> GPLGSSATPREDFRVRCTSKRAVTEMLQLCGRFVQKLGDALPEEIREPALRDAQWT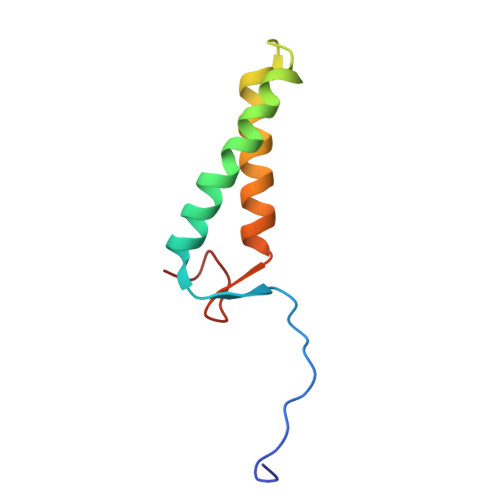FESAVQENISINGQAWQEAS>[3x]MLEANVYDNFNPNYYNISDFSMPNGKKEKRGLPIPKARCQVINYELWETGYLYTSSATLTVSVEVGDIVQILFPEVVPIEEALGKKKKLNLDMVYLVTDVDESNKATLKNYFWAMIESLDVPNAITKTTNFAIIDYLIDPNKNNLMSYGYFFNSSIFAGKATINRKAETSSAHDVAKRIFSKVQFQPTTTIQHAPSETDPRNLLFINFASRNWNRKRITTRVDIKQSVTMDTETIVERSAYNFAVVFVKNKATDDYTDPPKMYIAKNNGDVIDYSTYHGDGTDLPDVRTAKTLFYDRDDHGNPPELSTIKVEISPSTIVTRLIFNQNELLPLYVNDLVDIWYEGKLYSGYIADRVKTEFNDRLIFVESGDKPNVI;>[12x]MVRQYKIHTNLDGTDDKVWDVTNGKVRFYQPSNLGLQSTNNIWQSNGIGVMGTRSITQPQIEFKLETF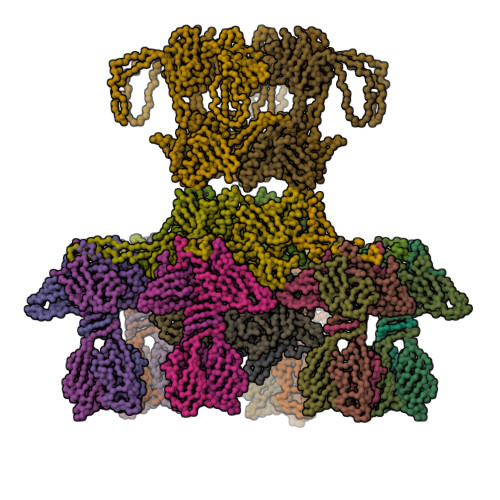GESLEENYQLMKDFVNDILSKKFVTLEYQTEIFQVYADLALADVTKTEGYGKNGTFSEKITFDIITKWYTYENLTFDKIQNGKVIAGMSKIYGGTAPGNYKYIKGTSYTYYGESDIDRLSRWDIKEEIFSFMGILYPKLPKTPAGVRFLDDIGNEYTAIVFKTEQVQDYILINTDVNDETYQGWKGTTALNLFPVMDFERYRTRIIEKGQMELINLSKAEFKIKRKADFV;>MTIKNFTFFSPNSTEFPVGSNNDGKLYMMLTGMDYRTIRRKDWSSPLNTALNVQYTNTSIIAGGRYFELLNETVALKGDSVNYIHANIDLTQTANPVSLSAETANNSNGVDINNGSGVLKVCFDIVTTSGTGVTSTKPIVQTSTLDSISVNDMTVSGSIDVPVQTLTVEAGNGLQLQLTKKNNDLVIVRFFGSVSNIQKGWNMSGTWVDRPFRPAAVQSLVGHFAGRDTSFHIDINPNGSITWWGANIDKTPIATRGNGSYFIK[18x]> MAARTSFL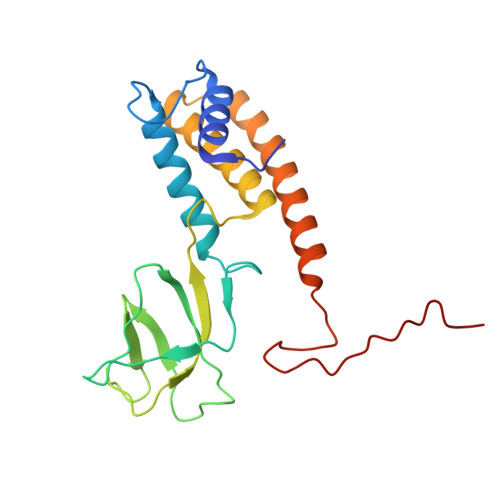DAVNRVLQMLGEAPVNSLQGQFGLAKQAEVALNDVSRTIQTEGWSFNTDLEKKLERNSSNEIELSSNVSRVVVDNLEYPDIDVVQRGDKLYDRKNNRYTFDEDLIVDMTTILEWDLLPEHARQYITIKAGRQLQEAIIGSAELTKLNLTQEVEARSAFLEEETTKSEHSMLRGHLNRTSPVNTYIPSRTLER The ABC-type transporter (NikABCDE) imports the metal from the extracellular environment through a multi-step process in many bacteria, including Enterobacteriaceae and S. aureus. While a bacterial nickelophore dedicated to the NikABCDE system is currently unknown, exogenous environmental l-histidine is believed to be a widespread ligand. l-Histidine forms Ni-(l-His)2 complexes, which exhibit a strong affinity for NikA for efficient transport into the cell through the NikBCDE ABC-type transporter. Previously, we identified that the fungal-derived polycarboxylic acid natural product aspergillomarasmine A (AMA) is a non-antimicrobial metallophore with a preference for Zn2+, Co2+, and Ni2+ ions. AMA-metal complexes target the periplasmic Ni2+ uptake protein NikA through high-affinity interactions and compete with Ni-(l-His)2 for uptake.

E. coli NikA (22-524), which shares 75% identity and 90.5% similarity with the K. pneumoniae ortholog, was purified for crystallization studies. Ni-AMA adopted different coordination geometry when bound to NikA compared to the stand-alone structure determined in our previous work, indicating that two configurations of the Ni-AMA complex are possible. Superposition of the Ni-AMA structures showed that relative to AMA’s l-Asp unit (l-AspAMA), the penultimate APA2 and N-terminal APA1 are rotated by 93.3°. The interaction network between NikA and Ni-AMA revealed that the conserved His416 residue occupies the axial position within the Ni-AMA complex. This observation suggests that NikA either conformationally selects for one form of Ni-AMA or that Ni-AMA binding to NikA induces a conformational change to accommodate the Ni2+ interaction with His416. The remainder of the ligand binding pocket of NikA around the Ni-AMA is composed of Tyr22, Met27, Trp100, Tyr382, Trp398, and Tyr402. Notable CH-π stacking interactions occur between Trp100 and APA2, and APA1 and Tyr382. Extensive electrostatic interactions also occur with the carboxyl groups of Ni-AMA, including hydrogen bonds with the side chain of Arg137 to the α-carboxyl of the l-AspAMA residue. Ni-AMA induced the closed conformation of NikA. The structure of the NikA:Ni-AMA complex shows that AMA metal complexes are reasonable Ni-(l-His)2 mimetics and that full NikA closure and high-affinity binding are likely facilitated by accepting His416 as the 6th Ni2+ ligand.

> APDEITTAWPVNVGPLNPHLYTPNQMFAQSMVYEPLVKYQADGSVIPWLAKSWTHSEDGKTWTFTLRDDVKFSNGEPFDAEAAAENFRAVLDNRQRHAWLELANQIVDVKALSKTELQITLKSAYYPFLQELALPRPFRFIAPSQFKNHETMNGIKAPIGTGPWILQESKLNQYDVFVRNENYWGEKPAIKKITFNVIPDPTTRAVAFETGDIDLLYGNEGLLPLDTFARFSQNPAYHTQLSQPIETVMLALNTAKAPTNELAVREALNYAVNKKSLIDNALYGTQQVADTLFAPSVPYANLGLKPSQYDPQKAKALLEKAGWTLPAGKDIREKNGQPLRIELSFIGTDALSKSMAEIIQADMRQIGADVSLIGEEESSIYARQRDGRFGMIFHRTWGAPYDPHAFLSSMRVPSHADFQAQQGLADKPLIDKEIGEVLATHDETQRQALYRDILTRLHDEAVYLPISYISMMVVSKPELGNIPYAPIATEIPFEQIKPV>GSHMRTEIDKPSQMQVTDVQDNSISVKWLPSSSPVTGYRVTTTPKNGPGPTKTKTAGPDQTEMTIEGLQPTVEYVVS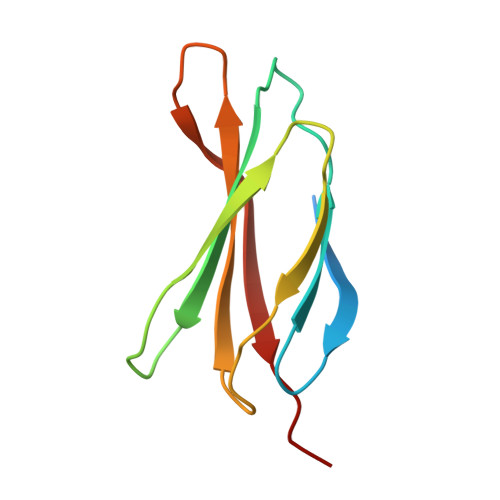VYAQNPSGESQPLVQTAVTTIPAP[10x]alpha-methyl-L-serine | C4 H9 N O3 | 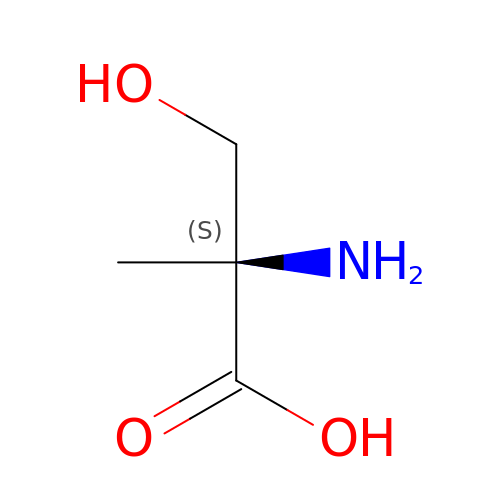CDUUKBXTEOFITR-BYPYZUCNSA-N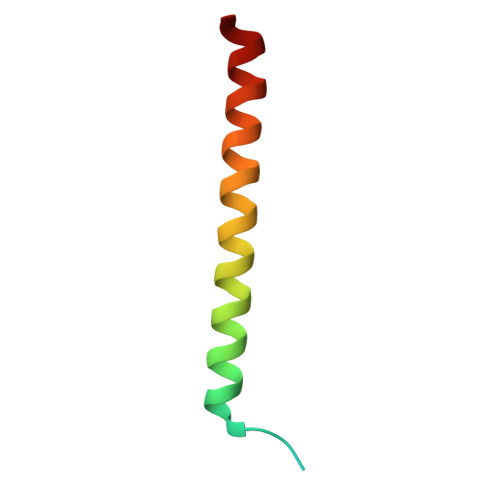> MNHFGAVKSEEKYYIDADLLREIKQHLKQQQEGLSHLISIIKDDLEDIKLV> ASMTGGQQMGRDQAGITGTWYNQLGSTFIVTAGADGA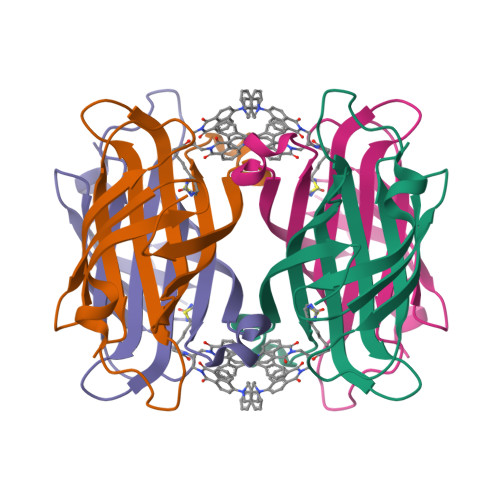LTGTYESAVGNAESRYVLTGRYDSAPATDGSGTALGWTVAWKNNYRNAHSATTWSGQYVGGAEARINTQWLLTSGTTEANAWKSTLVGHDTFTKVKPSAASIDAAKKAGVNNGNPLDAVQQ Abortive infection (Abi) is a bacterial antiphage defense strategy involving suicide of the infected cell. Some Abi pathways involve polymerases that are related to reverse transcriptases. They are unique in the way they combine the ability to synthesize DNA in a template-independent manner with protein priming. Here, we report crystal and cryo-electron microscopy structures of two Abi polymerases: AbiK and Abi-P2. Both proteins adopt a bilobal structure with an RT-like domain that comprises palm and fingers subdomains and a unique helical domain.

The structure of Ll-AbiK was determined by single-particle cryo-EM at 2.3 Å resolution. The Ll-AbiK hexamer is composed of two trimers that are stacked back-to-back, with the palm subdomains facing inward. In line with D3 symmetry of the hexamer, the two trimers are rotated relative to each other by 60° around a central three-fold axis of the trimer. The arrangement of the subunits creates a spherical cavity in the central part of hexamer with a diameter of ∼40 Å. Similarly, in the cryo-EM reconstruction two separate fragments of the DNA product can be seen—three nucleotides of the 5′ portion of the DNA, including the terminal nucleotide that is covalently attached to the protein, and eight nucleotides of the 3′ fragment that are accommodated within the channel. This implies that the region connecting these fragments is mobile or the DNA length could vary among individual molecules. In the cryo-EM structure of Ll-AbiK a clearly defined density of a 3′ nucleotide connected to the rest of the DNA is visible at the active site. The position of this nucleotide corresponds to the pre-translocation product state in which the last residue of the DNA occupies the position of the incoming nucleotide in substrate state. However, the position of the 3′ terminal nucleotide of the pre-translocation state captured in the Ll-AbiK-DNA structure is identical to the position of the incoming nucleotide in RNA/DNA complexes of the maturase and HIV-1 RT, reflecting the conservation of active site architecture.

>[6x]GSMKKEFTELYDFIFDPIFLVRYGYYDRSIKNKKMNTAKVELDNEYGKSDSFYFKVFNMESFADYLRSHDLKTHFNGKKPLSTDPVYFNIPKNIEARRQYKMPNLYSYMALNYYICDNKKEFIEVFIDNKFSTSKFFNQLNFDYPKTQEITQTLLYGGIKKLHLDLSNFYHTLYTHSIPWMIDGKSASKQNRKKGFSNTLDTLITACQYDETHGIPTGNLLSRIITELYMCHFDKQMEYKKFVYSRYVDDFIFPFTFENEKQEFLNEFNLICRENNLIINDNKTKVDNFPFVDKSSKSDIFSFFENITSTNSNDKWIKEISNFIDYCVNEEHLGNKGAIKCIFPVITNTLKQKKVDTKNIDNIFSKRNMVTNFNVFEKILDLSLKDSRLTNKFLTFFENINEFGFSSLSASNIVKKYFSNNSKGLKEKIDHYRKNNFNQELYQILLYMVVFEIDDLLNQEELLNLIDLNIDDYSLILGTILYLKNSSYKLEKLLKKIDQLFINTHANYDVKTSRMAEKLWLFRYFFYFLNCKNIFSQKEINSYCQSQNYNSGQNGYQTELNWNYIKGQGKDLRANNFFNELIVKEVWLISCGENEDFKYLN>MEIPSKQIDYRDVFIEFLTTFKGNNNQNKYIERINELVAYRKKSLIIEFSDVLSFNENLAYEIINNTKIILPILEGALYDHILQLDPTYQRDIEKVHVRIVGIPRVIELRKIRSTDIGKL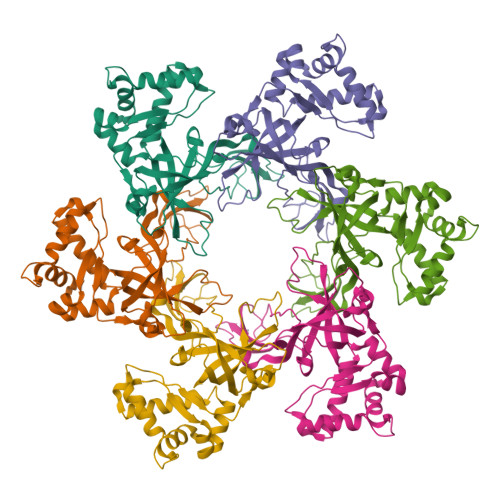ITIDGILVKVTPVKERIYKATYKHIHPDCMQEFEWPEDEEMPEVLEMPTICPKCGKPGQFRLIPEKTKLIDWQKAVIQERPEEVPSGQLPRQLEIILEDDLVDSARPGDRVKVTGILDIKQDSPVKRGSRAVFDIYMKVSSIEVSQKV[3x]>MTSIIKIDLESKTPIYKQIADQIIELIAKGELKPGDKLPSIRELASMLGVNMLTVNKAYNYLVD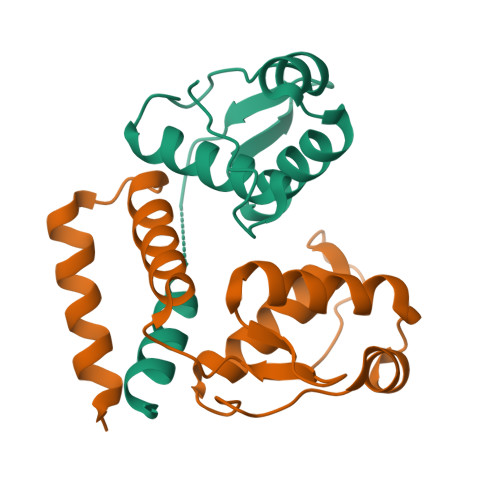EGFIVVQKRRYVVKSEVRDESWRNMLRVIIYRALASNMSKDEIVNEINRVVSEVNSK[2x]> MNIESSFCPILCICMIFLCLPNLSASQRCNNNDKQALLQIKTALKNPTITDSWVSDDDCCGWDLVECDETSNRIISLIIQDDEALTGQIPPQVGDLPYLQALWFRKLPNLFGKIPEEISALKDLKSLRLSSTSLSGPVPLFFPQLTKLTC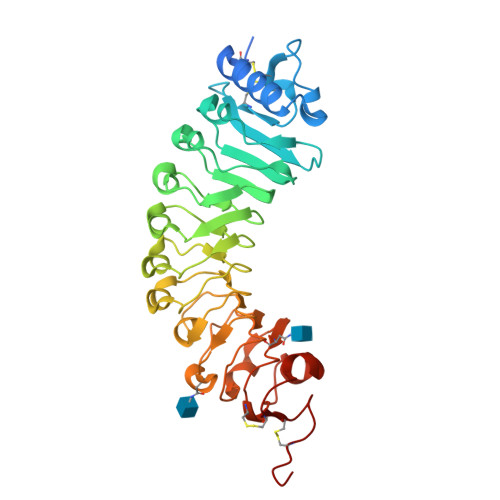LDLSFNKLLGVIPPQLSTLPNLKALHLERNELTGEIPDIFGNFAGSPDIYLSHNQLTGFVPKTFARADPIRLDFSGNRLEGDISFLFGPKKRLEMLDFSGNVLSFNFSRVQEFPPSLTYLDLNHNQISGSLSSELAKLDLQTFNVSDNNLCGKIPTGGNLQRFDRTAYLHNSCLCGAPLPECAAAA2-nitro-5-(phenylsulfonyl)phenol 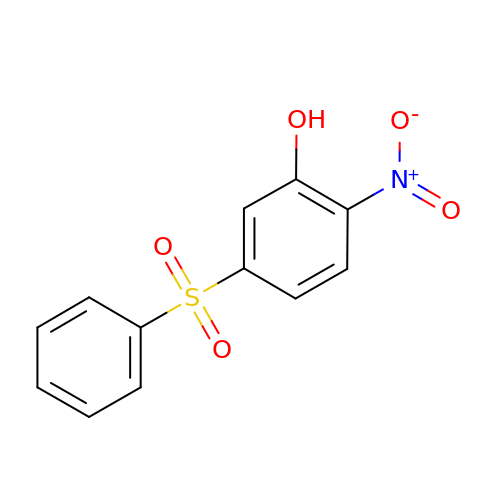| C12 H9 N O5 S | MPJBDZGASMKZSN-UHFFFAOYSA-N Aerobic arsenite oxidation is catalysed by arsenite oxidase (Aio) which is thought to be an ancient bioenergetic enzyme that was present in the last universal common ancestor prior to the divergence of the Bacteria and Archaea. Aio consists of two heterologous subunits, a large (93 kDa) catalytic subunit (AioA) which contains the molybdenum cofactor (Moco) at the active site and a 3Fe-4S cluster, and a small subunit (14 kDa) subunit (AioB) which contains a Rieske 2Fe-2S cluster. The Aio belongs to the dimethylsulphoxide (DMSO) reductase enzyme family of molybdoenzymes but is unusual in that it’s the only member of this family to contain a 3Fe-4S cluster and a Rieske subunit. Since the 3Fe-4S cluster is a one electron acceptor it is assumed that it accepts one electron from the Mo-pterin and then transfers an electron at a time to the Rieske 2Fe-2S cluster of the AioB subunit.

In this study, we report the first heterologous expression and X-ray crystal structure of the arsenite oxidase from the autotrophic arsenite-oxidising bacterium NT-26. The structure of the NT-26 Aio was solved to a resolution of 2.7 Å. The asymmetric unit of arsenite oxidase contains four α and four β chains. The same analysis reveals that the four heterodimers present in the asymmetric unit are arranged as two stable heterotetramers, and each heterotetramer buries 22000 Å2 of surface area (meaning the tetramerisation buries a further 6000 Å2 of surface area). The heterodimer of NT-26 (α and β subunits) superimposes with A. faecalis (1 g8j), 948 matching residues with an rmsd of 1.84 Å for cα atoms (the values for the individual chains are around 1 Å). The Mo metal sits in a five coordinate environment; four ligands come from the two dithiolene moieties, each of which comes from a pterin molecule. The fifth site is occupied by an oxygen (presumably an oxo group) giving rise to a square pyramidal arrangement of the five ligands. There is no evidence in the NT-26 Aio for a sixth ligand to the Mo centre. Another distinct feature of the NT-26 AioB Rieske structure is the absence of the disulphide bridge (C65–C80, A. faecalis numbering) shielding the cluster from solvent exposure. In NT-26 the aromatic ring of β F108 closes over the cluster packing against β G123, and could thus play the role of the shield.

>MAFKRHIDRLPIIPADAKKHNVTCHFCIVGCGYHAYTWPINKQGGTDPQNNIFGVDLSEQQQAESDAWYSPSMYNVVKQDGRDVHVVIKPDHECVVNSGLGSVRGARMAETSFSEARNTQQQRLTDPLVWRYGQMQPTSWDDALDLVARVTAKIVKEKGEDALIVSAFDHGGAGGGYENTWGTGKLYFEAMKVKNIRIHNRPAYNSEVHGTRDMGVGELNNCYEDAELADTIVAVGTNALETQTNYFLNHWIPNLRGESLGKKKELMPEEPHEAGRIIIVDPRRTVTVNACEQTAGADNVLHLAINSGTDLALFNALFTYIADKGWVDRDFIDKSTLREGTARPPLYPARGVSEANPGHLSSFEDAVEGCRMSIEEAAEITGLDAAQIIKAAEWIGMPKEGGKRRRVMFGYEKGLIWGNDNYRTNGALVNLALATGNIGRPGGGVVRLGGHQEGYVRPSDAHVGRPAAYVDQLLIGGQGGVHHIWGCDHYKTTLNAHEFKRVYKKRTDMVKDAMSAAPYGDREAMVNAIVDAINQGGLFAVNVDIIPTKIGEACHVILPAATSGEMNLTSMNGERRMRLTERYMDPPGQSMPDCLIAARLANTMERVLTEMGDVGYAAQFKGFDWQTEEDAFMDGYNKNAHGGEFVTYERLSAMGTNGFQEPATGFTDGKIEGTQRLYTDGVFSTDDGKARFMDAPWRGLQAPGKQQQKDSHKYLINNGRANVVWQSAYLDQENDFVMDRFPYPFIEMNPEDMAEAGLKEGDLVEIYNDAGATQAMAYPTPTARRGETFMLFGFPTGVQGNVTSAGTNELIIPNYKQTWGNIRKISDAPRNVAHLSFKSKEYQSA[4x];>[4x]MSRCQNMVDIGRRQFLRGGALAAAGATAAVFGVGAPQARAATAAAGVEYPANRLANISELTLNEPLDVAYPDEDAAGVLLKLGTRVEGGVGPDGDIVGFSTICPHKGFPLSYSADNKTFNCPGHFSVFDPEKGGQQVWGQATQNLPQYVLRVADNGDIFAEGVDELIYGRLSNVL>[2x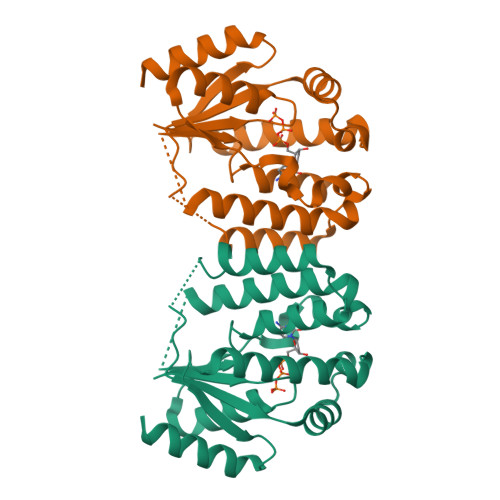]MKIAIFGTVGAGKSTISAEISKKLGYEIFKEPVEENPYFEQYYKDLKKTVFKMQIYMLTARSKQLKQAKNLENIIFDRTLLEDPIFMKVNYDLNNVDQTDYNTYIDFYNNVVLENLKIPENKLSFDIVIYLRVSTKTAISRIKKRGRSEELLIGEEYWETLNKNYEEFYKQNVYDFPFFVVDAELDVKTQIELIMNKLNSIKNPN>MTITLTENKRKSMEKLSVDGVISALAFDQRGALKRMMAQHQTKEPTVEQIEELKSLVSEELTPFASSILLDPEYGLPASRVRSEEAGLLLAYEKTGYDATTTSRLPDCLDVWSAKRIKEAGAEAVKFLLYYDIDGDQDVNEQKKAYIERIGSECRAEDIPFYLEILTYDEKIADNASPEFAKVKAHKVNEAMKVFSKERFGVDVLKVEVPVNMKFVEGFADGEVLFTKEEAAQAFRDQEASTDLPYIYLSAGVSAKLFQDTLVFAAESGAKFNGVLCGRATWAGSVKVYIEEGPQAAREWLRTE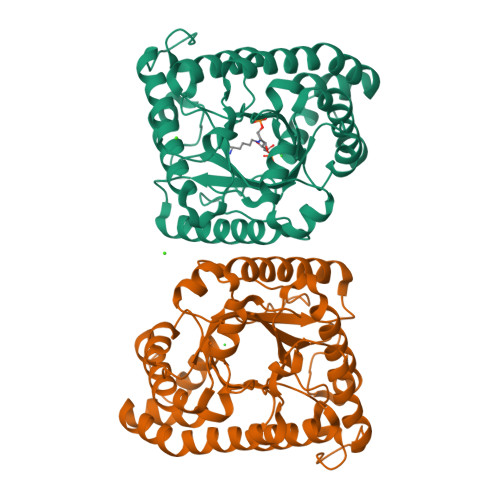GFKNIDELNKVLDKTASPWTEKM[4x]In response, one family of large bacteriophages uses a nucleus-like compartment to protect its replicating genomes by excluding host defence factors. Here we find that the bacteriophage nuclear shell assembles primarily from one protein, which we name chimallin (ChmA). Combining cryo-electron tomography of nuclear shells in bacteriophage-infected cells and cryo-electron microscopy of a minimal chimallin compartment in vitro, we show that chimallin self-assembles as a flexible sheet into closed micrometre-scale compartments. We find that the shell is primarily composed of a single protein, chimallin, which self-assembles through its extended N and C termini into a closed compartment.

Further reduction of the structure to focus on an individual protomer resulted in the highest quality map at about 3.1 Å resolution, enabling atomic modelling of the chimallin protomer. Chimallin folds into a compact two-domain core with extended N- and C-terminal segments. The N-terminal domain (residues 62–228) shows little structural homology to any characterized protein, adopting an αβ fold that is topologically similar only to an uncharacterized protein from Enterococcus faecalis. Although chimallin lacks the acetyltransferase active site residues of AtaT and related toxins, this structural similarity suggests that the jumbo phage nuclear shell may have evolved from a bacterial toxin–antitoxin system. The chimallin protomer map contains three interacting peptide segments from the N and C termini of neighbouring protomers. The N-terminal interacting segment (NTS: residues 48–61) of each protomer extends anticlockwise (as viewed from outside the cube) and docks against a neighbouring protomer’s N-terminal domain within a given face of the cubic assembly, thus establishing intra-tetramer connections. Two extended segments of the C terminus (CTS1: residues 590–611; and CTS2: residues 622–631) establish inter-tetramer interactions. Notably, the binding of CTS1 to the chimallin C-terminal domain resembles the interaction of the antitoxin AtaR with the AtaT acetyltransferase toxin, further hinting that the phage nuclear shell could have evolved from a bacterial toxin–antitoxin system.

>SNAMIRDTATNTTQTQAAPQQAPAQQFTQAPQEKPMQSTQSQPTPSYAGTGGINSQFTRSGNVQGGDARASEALTVFTRLKEQAVAQQDLADDFSILRFDRDQHQVGWSSLVIAKQISLNGQPVIAVRPLILPNNSIELPKRKTNIVNGMQTDVIESDIDVGTVFSAQYFNRLSTYVQNTLGKPGAKVVLAGPFPIPADLVLKDSELQLRNLLIKSVNACDDILALHSGERPFTIAGLKGQQGETLAAKVDIRTQPLHDTVGNPIRADIVVTTQRVRRNGQQENEFYETDVKLNQVAMFTNLERTPQAQAQTLFPNQQQVATPAPWVASVVITDVRNADGIQANTPEMYWFALSNAFRSTHGHAWARPFLPMTGVAKDMKDIGALGWMSALRNRIDTKAANFDDAQFGQLMLSQVQPNPVFQIDLNRMGETAQMDSLQLDAAGGPNAQKAAATIIRQINNLGGGGFERFFDHTTQPILERTGQVIDLGNWFDGDEKRDRRDLDNLAALNAAEGNENEFWGFYGAQLNPNLHPDLRNRQSRNYDRQYLGSTVTYTGKAERCTYNAKFIEALDRYLAEAGLQITMDNTSVLNSGQRFMGNSVIGNNMVSGQAQVHSAYAGTQGFNTQYQTGPSSFY[5x]> VHWTQEERDEISKTFQGTDMKTVVTQALDRMFKVYPWTNRYFQKRTDFRSSIHAGIVVGALQDAVKHMDDVKTLFKDLSKKHADDLHVDPGSFHLLTDCIIVELAYLRKDCFTPHI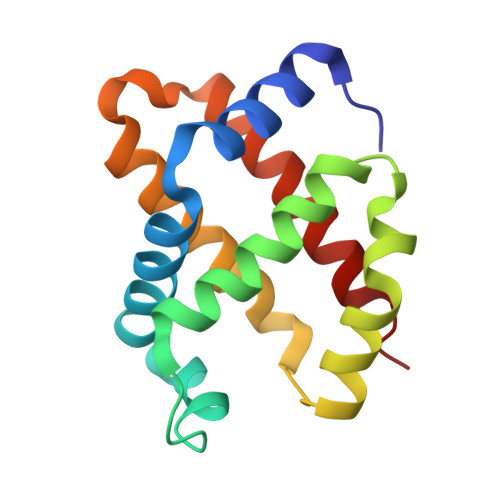QGIWDKFFEVVIDAISKQYH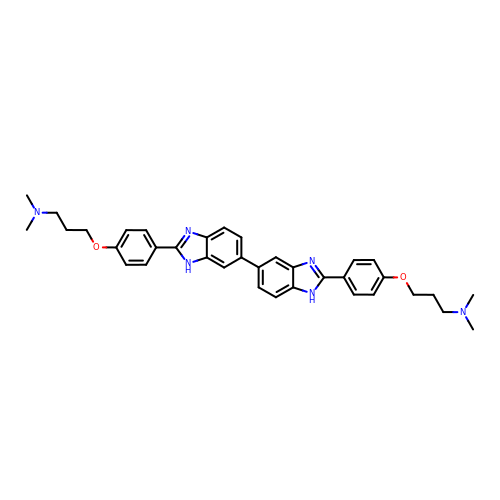[3-(4-{2'-[4-(3-DIMETHYLAMINO-PROPOXY)-PHENYL]-3H,3'H-[5,5']BIBENZOIMIDAZOLYL-2-YL}-PHENOXY)-PROPYL]-DIMETHYL-AMINE | C36 H40 N6 O2 | MZGMYDKOHYOXKR-UHFFFAOYSA-N>[10x]GRVDGQPMYGMESQVEEVRVFDTGVDAITEVECFLNPEMGDPDENLRGFSLKLSAENDFSSDSPERKMLPCYSTARIPLPNLNEDLTCGNLLM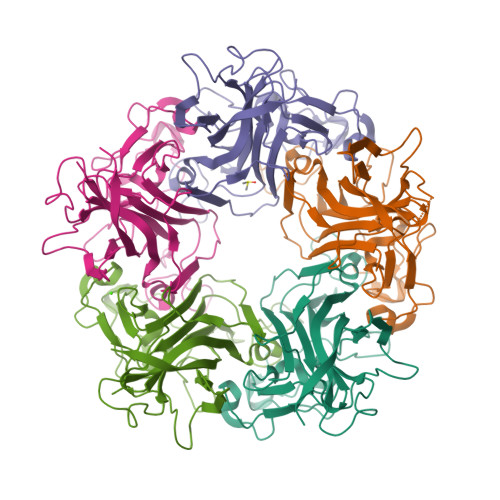WEAVTVQTEVIGITSMLNLHAGSQKVHEHGGGKPIQGSNFHFFAVGGEPLEMQGVLMNYRSKYPDGTITPKNPTAQSQVMNTDHKAYLDKNNAYPVECWVPDPSRNENARYFGTFTGGENVPPVLHVTNTATTVLLDEQGVGPLCKADSLYVSAADICGLFTNSSGTQQWRGLARYFKIRLRKRSVKNPY>MAHHHHHHMATPHNSAKVGDFAETVLMCGDPLRAKLIADNYLENAKQVNSVRGMLGFTGTYKGKPLSVMGHGMGIPSISIYAEELYNVYKVKTIIRVGTCGTVDPNVHVRDVCIVTASGTDSNVNRMRLLGHDFPATANFEVVSALVESAKALNIPTQVGKAYSTDIFYSKEQGLNEALAQ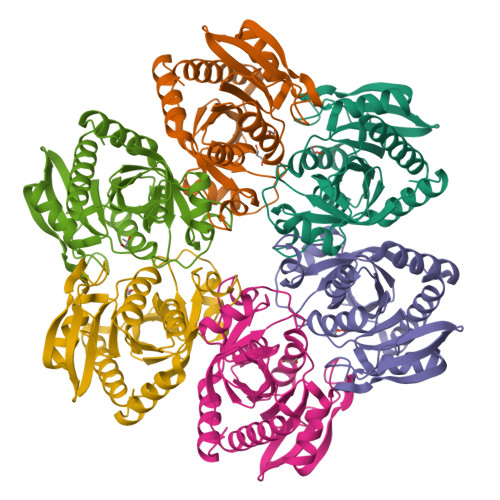YHFIAVEMESAGLFPIADYYGARAGCICTVSDHIITHESATPEERQTSFQNMIKIALEATLKL[6x]> ADFQGLYAEVKACSSELESLEMELRQQILVNIGKILQDQPSMEALEASLGQGLCSGGQVEPLDGPAGCILECLVLDSGELVPELAAPIFYL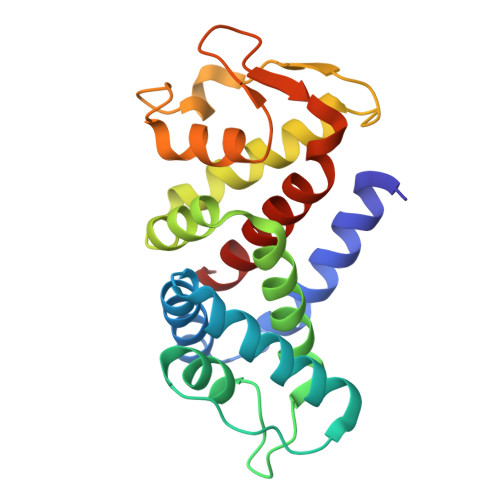LGALAVLSETQQQLLAKALETTVLSKQLELVKHVLEQSTPWQEQSSVSLPTVLLGDCWDEKNPTWVLLEECGLRLQVESPQVHWEPTSLIPTSALYASLFLLSSLGQ> GASAPIGAPTDVNVEPIGSRTLKVTWRPPLVDHWNGIIKGYYVGHK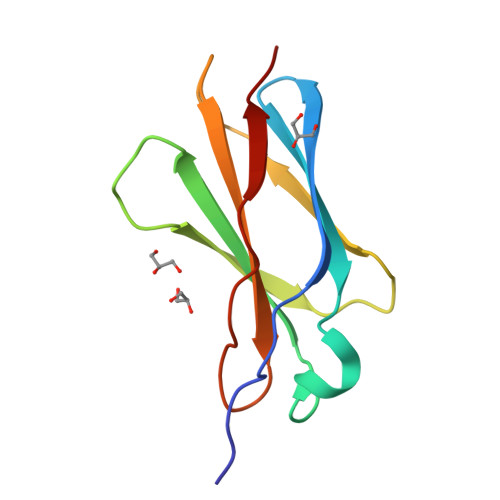ESDSSQQYRYQRVERSGINPETLLIAGLQKAKVYNVVVKAFNTAGSGPESHPVEAYSLE> AFSNQVIQRGASGEDVIELQSRLKYNGFYTG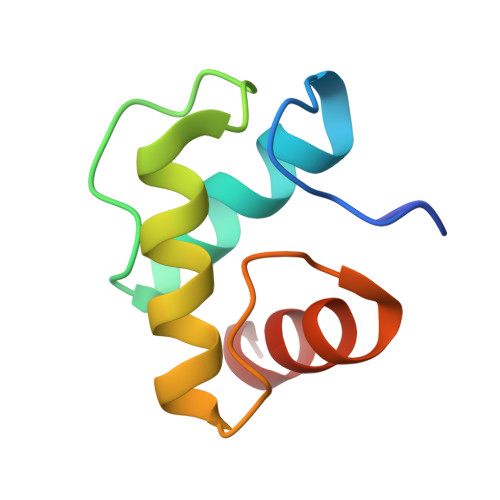KVDGVFGWGTYWALRNFQEKFGLPVDGLAGAKTKQMLVKATKY>[4x]MSYTVGTYLAERLVQIGLKHHFAVAGDYNLVLLDNLLLNKNMEQVYCCNELNCGFSAEGYARAKGAAAAVVTYSVGALSAFDAIGGAYAENLPVILISGAPNNNDHAAGHVLHHALGKTDYHYQLEMAKNITAAAEAIYTPEEAPAKIDHVIKTALREKKPVYLEIACNIASMPCAAPGPASALFNDEASDEASLNAAVEETLKFIANRDKVAVLVGSKLRAAGAEEAAVKFADALGGAVATMAAAKSFFPEENPHYIGTSWGEVSYPGVEKT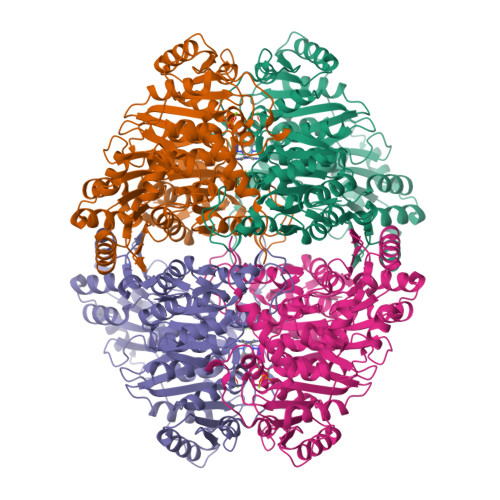MKEADAVIALAPVFNDYSTTGWTDIPDPKKLVLAEPRSVVVNGIRFPSVHLKDYLTRLAQKVSKKTGALDFFKSLNAGELKKAAPADPSAPLVNAEIARQVEALLTPNTTVIAETGDSWFNAQRMKLPNGARVEYEMQWGHIGWSVPAAFGYAVGAPERRNILMVGDGSFQLTAQEVAQMVRLKLPVIIFLINNYGYTIEVMIHDGPYNNIKNWDYAGLMEVFNGNGGYDSGAGKGLKAKTGGELAEAIKVALANTDGPTLIECFIGREDCTEELVKWGKRVAAANSRKPVNKLL>[2x]GCGSRAPIPEPKPGDLIEIFRPFYRHWAIYVGDGYVVHLAPDILLALTNDKERTQKVVSNKRLLLGVICKVAIVKKELLYDVAGSDKYQVNNKHDDKYSPLPCSKIIQRAEELV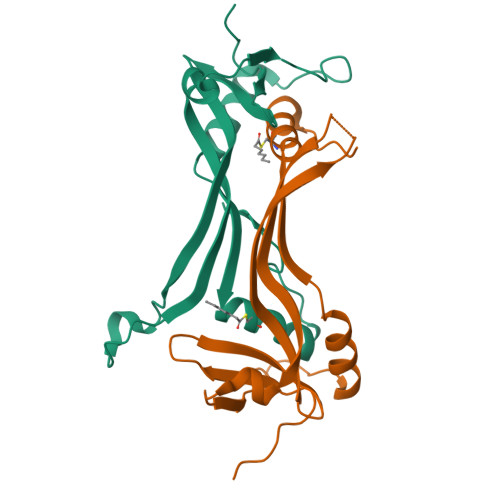GQEVLYKLTSENCEHFVNELRYGVARSDQEFIVTD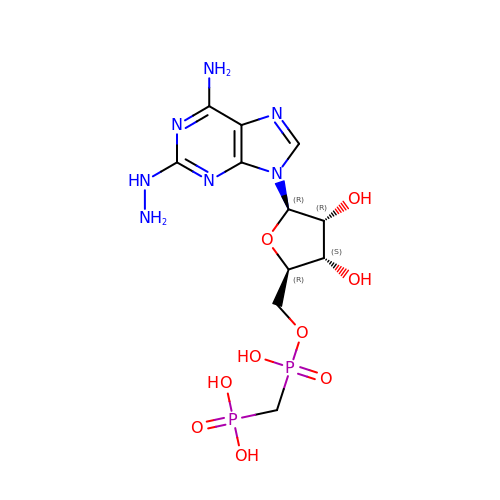[[(2~{R},3~{S},4~{R},5~{R})-5-(6-azanyl-2-diazanyl-purin-9-yl)-3,4-bis(oxidanyl)oxolan-2-yl]methoxy-oxidanyl-phosphoryl]methylphosphonic acid | C11 H19 N7 O9 P2 | AJMJEKNHUHCOGZ-KQYNXXCUSA-N> MSQPQSSQVTKRGLTDPERAAIIAAAVPDHALDTQRKYHYFIQPRWKRLSEYEQLSCYAQPNPDWIAGGLDWGDWTQKFHGGRPSWGNESTELRTTDWYRHRDPARRWHHPYVKDKSEEARYTQRFLAAYSSEGSIRTIDPYWRDEILNKYFGALLYSEYGLFNAHSSVGRDCLSDTIRQTAVFAALDKVDNAQMIQMERLFIAKLVPGFDASTDVPKKIWTTDPIYSGARATVQEIWQGVQDWNEILWAGHAVYDATFGQFARREFFQRLATVYGDTLTPFFTAQSQTYFQTTRGAIDDLFVYCLANDSEFGAHNRTFLNAWTEHYLASSVAALKDFVGLYAKVEKVAGATDRAGVSEALQRVFGDWKIDYAD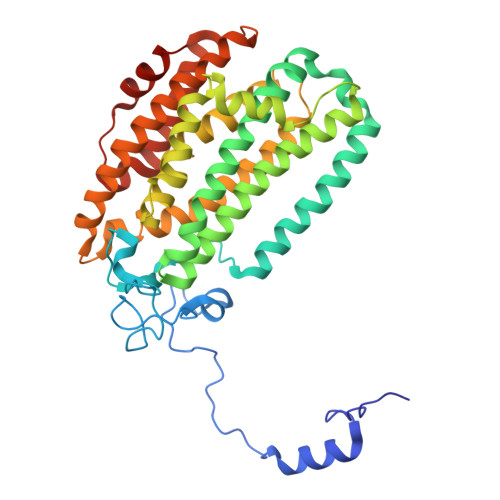KIGFRVDVDQKVDAVLAGYKN> GHMVTRIENLENAKKLWDNANSMLEKGNISGYLKAANELHKFMKEKNLKEDDLRPELSDKTISPKGYAILQSLWGAASDYSRAAATLTESTVEPGLV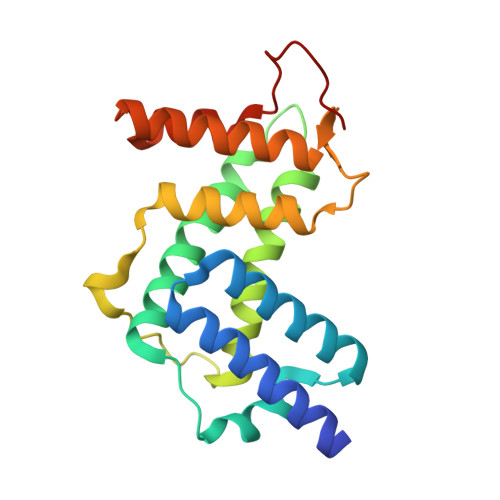SAVNKMSAFFMDCKLSPNERATPDPDFKVGKSKILVGIMQFIKDVADPTSKIWMHNTKALMNHKIAAIQKLERSNNVNCETLESVLSSKGENLSEYLSYK>[3x]MGQGPELHLASQFVNEACRALVFGGCVEKSSVSRNPEVPFESSAYRISASARGKELRLILSPLPGAQPQQEPLALVFRFGMSGSFQLVPREELPRHAHLRFYTAPPGPRLALCFVDIRRFGRWDLGGKWQPGRGPCVLQEYQQFRENVLRNLADKAFDRPICEALLDQRFFNGIGNYLRAEILYRLKIPPFEKARSVLEALQQHRPSPELTLSQKIRTKLQNPDLLELCHSVPKEVVQLGGRGYGSESGEEDFAAFRAWLRCYGMPGMSSLQDRHGRTIWFQGDPGPLAPKGRKS

Human endonuclease VIII-like 1 (hNEIL1) is a bifunctional DNA glycosylase of the Fpg/Nei family, which catalyzes the removal of damaged bases and subsequent incision of the newly generated abasic sites. Unlike traditional enzymes which are commonly referred to as highly specific biocatalysts, one special feature for hNEIL1 is its unique capability to recognize a wide range of substrates, including formamidopyrimidines, hydantoin lesions, oxidized, and dihydro-modified pyrimidine bases, derived from all four canonical bases. Here, by integrating structural, computational, and biochemical investigations, we show that hNEIL1 uses a triage mechanism to achieve broad specificity and reduce futile repair of normal bases. This mechanism involves two mutually competing interaction states: an activated state that commits catalysis and BER, and a quarantine state that temporarily separates and prevents the flipped base from catalysis via auto-inhibition.

For a naturally existing hNEIL1 variant (R242)14 in complex with dsDNAs containing OHU, Sp1, or Gh, the damaged bases are in close contact with the guanidine group of R242. Such conformation of the lesion recognition loop resembles that in the hNEIL1-Tg structure, where the positively charged side chain of residue 242 is contiguous to the solvent-exposed flipped base while the aromatic residue Y244 is laid away from the active site (thus called “242-in” conformation). Noteworthy, across all these structures, we observed an unusually short distance (~3.0 Å) between an outwards heterocyclic nitrogen atom of the nucleobases and the terminal nitrogen atom of residue 242. While repulsion is expected for the two groups if both are fully protonated (i.e., an −NH group in the nucleobase and a positively charged side chain of residue 242), we previously showed in the hNEIL1–Tg complex that hNEIL1 utilizes a tautomerization-dependent mechanism to recognize the flipped base. In this mechanism, the base undergoes a keto-enol tautomerization event where the originally protonated heterocyclic nitrogen atom becomes a hydrogen bond acceptor and hence can be hydrogen-bonded to residue 242. The fact that different recognition states were crystallographically captured for the same edited hNEIL1(R242) variant bound to different base lesions suggests that the flipped nucleobase per se also contributes to the stability of the interaction states. hNEIL1 repairs a diverse array of base damage, whose aromaticity and hydrophilicity differ greatly. Oxidized substrates of hNEIL1 are often bulky and contain non-planar structures; this disrupted aromaticity is expected to diminish the π–π stacking with Tyr244 and hence destabilize the quarantine state. Moreover, it is expected that the bases with less solvent interactions (e.g. DHU) would favor the formation of a stable quarantine state compared with the hydrophilic bases (Sp1, 5-OHU, Gh, and Tg).> MMTGTIETTGNISAEKGGSIILQCHLSSTTAQVTQVNWEQQDQLLAISN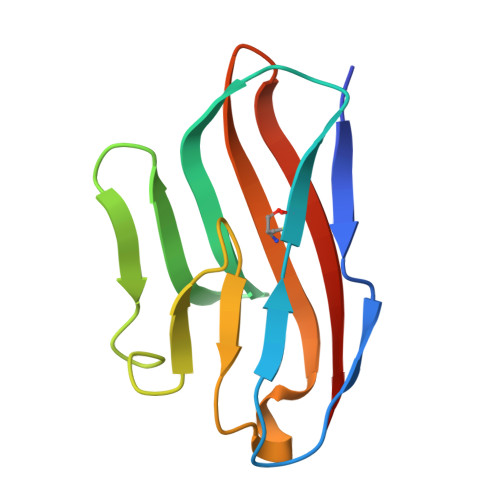ADLGWHISPSFKDRVAPGPGLGLTLQSLTVNDTGEYFCIYHTYPDGTYTGRIFLEVLE>XGC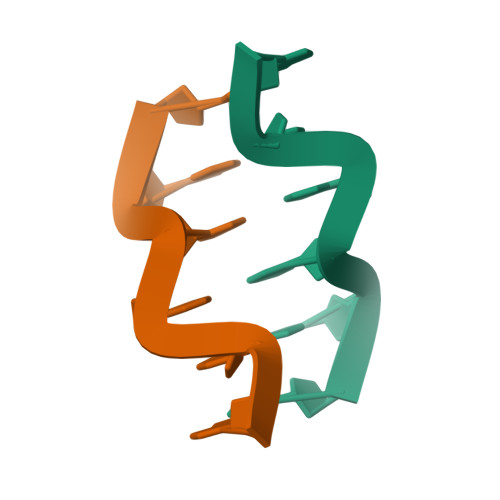GCG[2x]> ASSTNLKDVLAALIPKEQARIKTFRQQHGGTALGQITVDMSYGGMRGMKGLVYETSVLDPDEGIRFRGFSIPECQKLLPKGGXGGEPLPEGLFWLLVTGQIPTGAQVSWLSKEWAKRAALPSHVVTMLDNFPTNLHPMSQLSAAITALNSESNFARAYAEGILRTKYWEMVYESAMDLIAKLPCVAAKIYRNLYRAGSSIGAIDSKLDWSHNFTNMLGYTDAQFTELMRLYLTIHSDHEGGNVSAHTSHLVGSALSDPYLSFAAAMNGLAGPLHGLANQEVLGWLAQLQKAXXXAGADASLRDYIWNTLNSGRVVPGYGHAVLRKTDPRYTCQREFALKHLPGDPMFKLVAQLYKIVPNVLLEQGAAANPWPNVDAHSGVLLQYYGMTEMNYYTVLFGVSRALGVLAQLIWSRALGFPLERPKSMSTDGLIAL;> ASSTNLKDVLAALIPKEQARIKTFRQQHGGTALGQITVDMSYGGMRGMKGLVYETSVLDPDEGIRFRGFSIPECQKLLPKGGGGEPLPEGLFWLLVTGQIPTGAQVSWLSKEWAKRAALPSHVVTMLDNFPTNLHPMSQ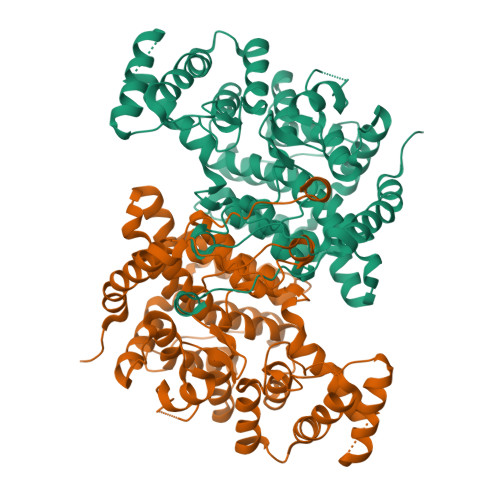LSAAITALNSESNFARAYAEGILRTKYWEMVYESAMDLIAKLPCVAAKIYRNLYRAGSSIGAIDSKLDWSHNFTNMLGYTDAQFTELMRLYLTIHSDHEGGNVSAHTSHLVGSALSDPYLSFAAAMNGLAGPLHGLANQEVLGWLAQLQKAAGADASLRDYIWNTLNSGRVVPGYGHAVLRKTDPRYTCQREFALKHLPGDPMFKLVAQLYKIVPNVLLEQGAAANPWPNVDAHSGVLLQYYGMTEMNYYTVLFGVSRALGVLAQLIWSRALGFPLERPKSMSTDGLIAL>[4x]TGVFGGYSERANHQANPEF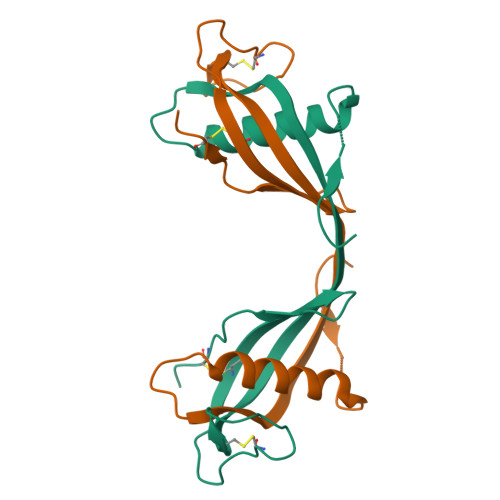LNLAHYATSTWSAQQPGKTHFDTVAEVVKVETQVVAGTNYRLTLKVAESTCELTSTYNKDTCLPKADAAHRTCTTVVFENLQGDKSVSPFECEAA> PLGSMSDRDVCIQRLTGANQDHILTALEHGSEAERASLTAQITNELAGVDFRHFNDVLRESLEISKNCSTASLAEPPAKDSFFDISSVDRRRGQAKRIKNLEAVGYKAIQKGQIAFLILAGGSGTRLGFDKPKGFFTCDGLQQRKSLFMMHCEKIRRRQEIAESISGSGRKARVQLLVMTSGQNDAETQRFFEENSYFGLEREQVHFFAQSSVPCYDENTGRIIMENRGRICAAPGGNGAVFAALAAPRATKDKDGTLQVKESLLQHLRKLGIAYVQIGNIDNLLANVADPVFIGYAIEEEAHVVVKTCPKRGPDERVGVFVRASGKWGVVEYTEIGDRAKEIDDATGELKFNCANISSNLCSLHFMSLAAERMKSFTQYHAARKKIPTIKGPVMGIKLEAFLFDLFRFVDECDHPPKDSGAFRIMQVDRDDEFGPVKNADGAASDTPADAVRLLLSQHTRWLITALETAAMSDEQESIRGGVDVTEAKEAVAVMRSCSIKAEISPLVSVGGEGLRQHLPRVIHQLLRNPPPVIFIRRD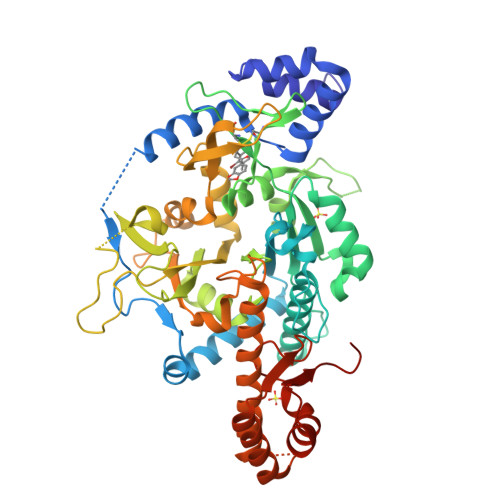DEVVSESSNM> MGFHFQQYIAMAGRAINPVQWTRAWRRMEGKSATEVYR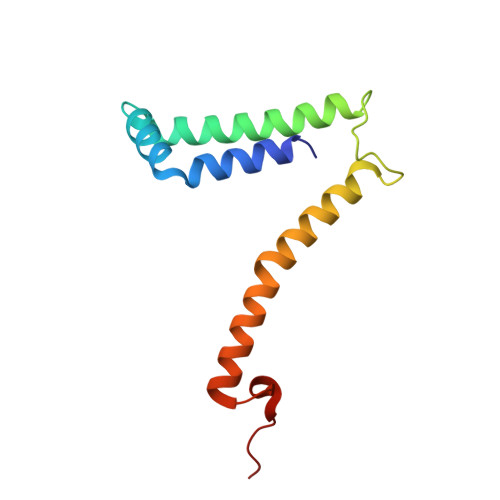DALAWTNNQFAQISRASQYRAWWWQNPLGMGLVLYGTYKAWHMIYMVRKQKKTAQLVAAAYGQGGQWLNPVPR A 60-kDa FAD-dependent oxidoreductase, AIF allosterically switches between two distinct redox states. NADH binding by the oxidized AIF monomer reduces its FAD cofactor at a centralized active site, allosterically disrupting hydrogen bond networks to release a 50-residue surface loop (C-loop) and stimulate dimerization at the AIF surface. Oxidized NAD+ and reduced FADH– form a long-lived charge-transfer complex (CTC), which stabilizes and maintains the reduced dimeric state of AIF. NADH-activated AIF dimers support import of OXPHOS subunits by CHCHD4 and are critical for mitochondrial function.

To understand how SAXS CX1 and CX2 chemotypes engage AIF and enable dimerization, we crystallized select fragment hits with the W196A dimer-permissive mutant and wild-type AIF. Crystal structures of the W196A mutant bound to CX1 fragments and the underlying 4-aminoquinoline (4AQ) scaffold revealed that these scaffolds localize to the NADH active site, mirroring the native NADH ligand, as do CX1 and CX2 scaffolds bound to the wild-type protein. In all four W196A structures, the CX1 quinoline core aromatically pairs with the AIF FAD cofactor, positioning the primary amine to hydrogen bond with the E314 side-chain carboxylate and the W483 backbone carbonyl. To accommodate this amine interaction, the aromatic side chain of F482 must rotate out of the binding site. In AIF structures with NADH and CX1 fragments, the released H454 imidazole ring is well positioned to aromatically contact and retain the displaced phenylalanine ring of F482, thus allowing access to W483 and E314 contact sites. Halogen substitutions at positions 7 and 8 (fragments C12, D1 and D3) optimally accelerate dimerization. By contrast, the complementary chlorine-substituted analogs D3 and D1 with slower kVR rates do not make analogous halogen-π contacts, presumably from steric restriction of the larger chlorine atom. They still form optimal amine hydrogen bonds with the active site, and the aromatic edge at positions 2 and 3 is aligned to form edge contacts with F482 and H454 aromatic rings. When the AIF(W196A) mutant is co-incubated with CX1 fragments, the oxidized mutant fully dimerizes and remains dimeric throughout the time series, similar to the wild-type AIF–NADH–DMSO control. The ability of the CX1 chemotype to shift the dimer-permissive W196A mutant toward the dimeric state also implicates F482 displacement and H454–F482 pairing in allosterically stabilizing the AIF dimer.

>[2x]MVGAGAYAYKTMKEDEKRYNERISGLGLTPEQKQKKAALSASEGEEVPQDKAPSHVPFLLIGGGTAAFAAARSIRARDPGARVLIVSEDPELPYMRPPLSKELWFSDDPNVTKTLRFKQANGKERSIYFQPPSFYVSAQDLPHIENGGVAVLTGKKVVQLDVRDNMVKLNDGSQITYEKCLIATGGTPRSLSAIDRAGAEVKSRTTLFRKIGDFRSLEKISREVKSITIIGGGFLGSELACALGRKARALGTEVIQLFPEKGNMGKILPEYLSNWTMEKVRREGVKVMPNAIVQSVGVSSGKLLIKLKDGRKVETDHIVAAVGLEPNVELAKTGGLEIDSDFGGFRVNAELQARSNIWVAGDAACFYDIKLGRRRVEHHDHAVVSGRLAGENMTGAAKPYWHQSMFWSDLGPDVGYEAIGLVDSSLPTVGVFAKATAQDNPKSATEQSGTGIRSESETESEASEITIPPSTPAVPQAPVQGEDYGKGVIFYLRDKVVVGIVLWNIFNRMPIARKIIKDGEQHEDLNEVAKLFNIHEDLEVLFQ> SNAMSNANQKITTFLMFEGKAEEAMNFYTSLFDQSEIVSISRYDENGPGKEGTVIHATFTLNGQEFMCIDSYVNHNFTFTPAMSLYVTCETEEEIDTVFHKLAQDGAILMPLGSYPFSKKFGWLNDKYGVS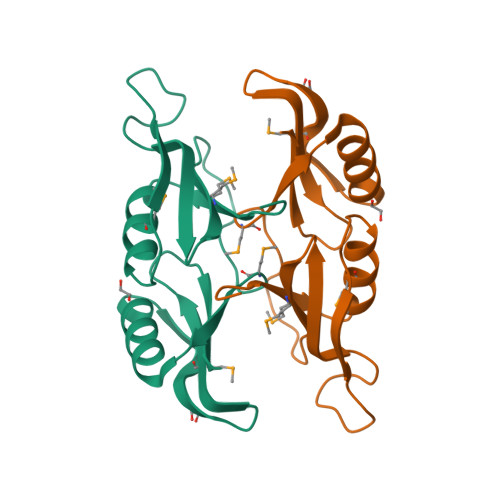WQLTLAE GUANYLYL-2',5'-PHOSPHOGUANOSINE | C20 H25 N10 O12 P | 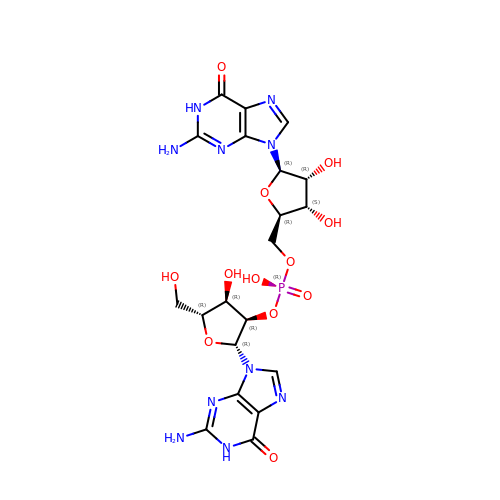YYNDAHWXMRBBRC-MHARETSRSA-N>MSIPVTEFRQFSEQQPAFRVLKPWWDVFTDYLSVAMLMIGVFGCTLQVMQDKIICLPKRVQPAQNHSSLSNVSQAVASTTPLPPPKPSPANPITVEMKGLKTDLDLQQYSFINQMCYERALHWYAKYFPYLVLIHTLVFMLCSNFWFKFPGSSSKIEHFISILGKCFDSPWTTRALSEVSGEDSEEKDNRKNNMNRSNTIQSGPEGSLVNSQSLKSIPEKFVVDKSTAGALDKKEGEQAKALFEKVKKFRLHVEEGDILYAMYVRQTVLKVIKFLIIIAYNSAL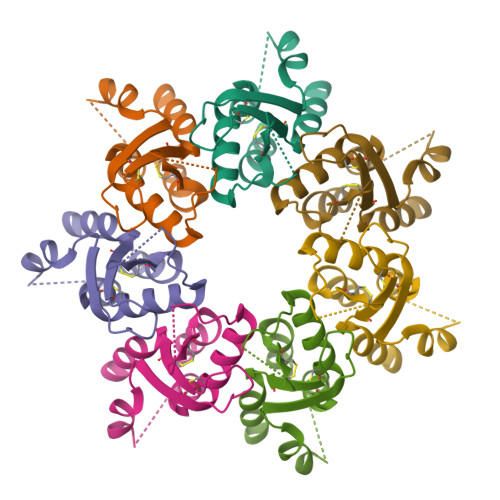VSKVQFTVDCNVDIQDMTGYKNFSCNHTMAHLFSKLSFCYLCFVSIYGLTCLYTLYWLFYRSLREYSFEYVRQETGIDDIPDVKNDFAFMLHMIDQYDPLYSKRFAVFLSEVSENKIKAAELKALEVLFQ[7x]> G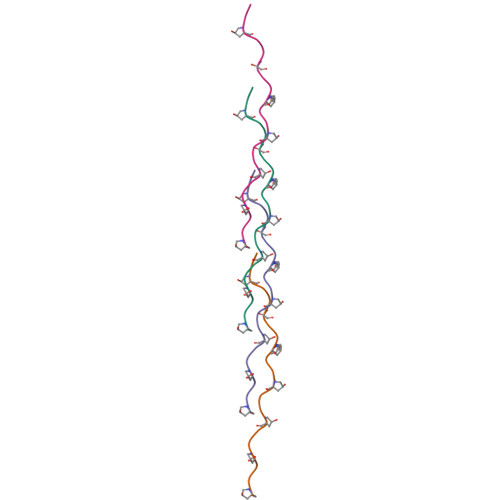PPGPPGPPGPPGPPGPPGPPGPPGPPGPP> MKTSDANETEDHLESLICKVGEKSACSLESNLEGLAGVLEADLPNYKSKILRLLCTVARLLPEKLTIYTTLVGLLNARNYNFGGEFVEAMIRQLKESLKANNYNEAVYLVRFLSDLVNCHVIAAPSMVAMFENFVSVTQEEDVPQVRRDWYVYAFLSSLPWVGKELYEKKDAEMDRIFANTESYLKRRQKTHVPMLQVWTADKPHPQEEYLDCLWAQIQKLKKDRWQERHILRPYLAFDSILCEALQHNLPPFTPPPHTEDSVYPMPRVIFRMFDYTDDPEGPVMPGSHSVERFVIEENLHCIIKSHWKERKTCAAQLVSYPGKNKIPLNYHIVEVIFAELFQLPAPPHIDVMYTTLLIELCKLQPGSLPQVLAQATEMLYMRLDTMNTTCVDRFINWFSHHLSNFQFRWSWEDWSDCLSQDPESPKPKFVREVLEKCMRLSYHQRILDIVPPTFSALCPVNPTCIYKYGDESSNSLPGHSVALCLAVAFKSKATNDEIFSILKDVPNPNQDDDDDEGFSFNPLKIEVFVQTLLHLAAKSFSHSFSALAKFHEV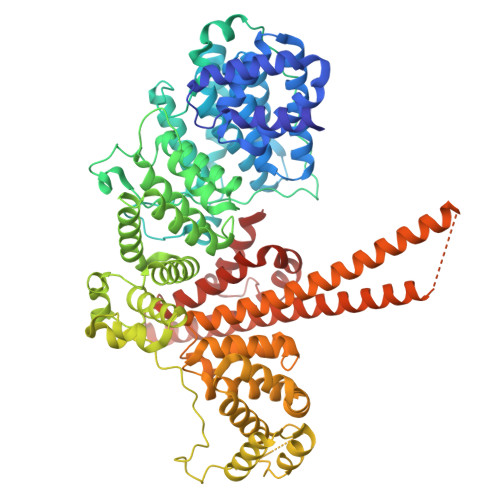FKTLAESDEGKLHVLRVMFEVWRNHPQMIAVLVDKMIRTQIVDCAAVANWIFSSELSRDFTRLFVWEILHSTIRKMNKHVLKIQKELEEAKEKLARQHKRRSDDDDRSSDRKDGVLEEQIERLQEKVESAQSEQKNLFLVIFQRFIMILTEHLVRCETDGTSVLTPWYKNCIERLQQIFLQHHQIIQQYMVTLENLLFTAELDPHILAVFQQFCALQA>MQAKIENPLKSLKTALNKIVLVKLKNGEEYVGRLEQSDGTMNLVLKDCTEYREGTSDPVAKYGRVLIRGSN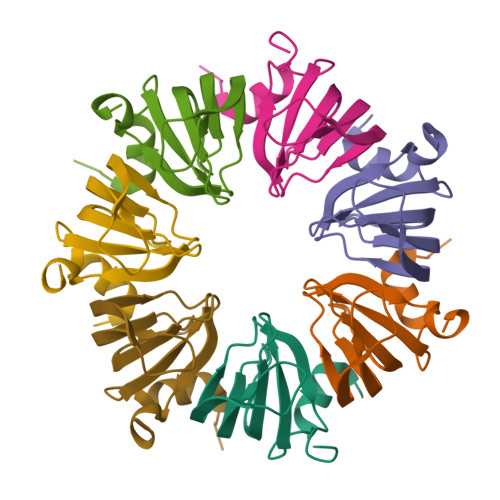ILFISIDYESIMGKEK[28x]>[2x]GSKNLIGRHLRLGSVEEQPFMFFATEGCEGNDCWSGMVNDMVVKLSEDLGFTYEYIQPDDRKFGALNKTTNEWNGMIRDLLDDKTDMIAIDLSTNSARKSAIDYSFPFMDAGIKAVVKGEGTTLNQVLELLDQDKYKWGVIGSKHPETLLKTHRDSRYSRLVDEGVELKDLNHAIETLRGGLFVFIDEGPVLAHNLISDCDVFSVGEEFQSFEYAFGLPKDSPYKSLIDSHLLKFREEGFI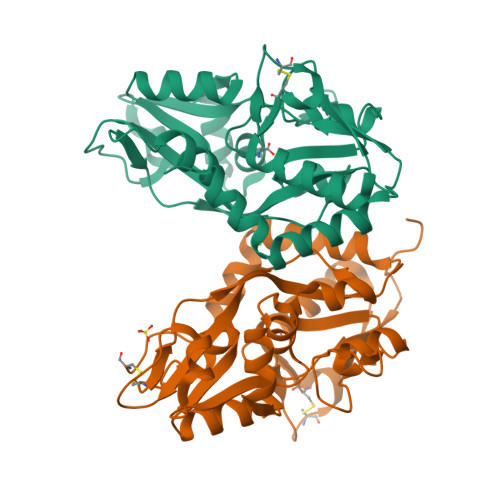DILWEKWSSGNSVCS Polycomb Repressive Complex 2 (PRC2) is a histone methyltransferase complex composed of core subunits Ezh2 (or Ezh1), Eed, Suz12 and Rbbp4. PRC2 trimethylates histone H3K27 (H3K27me3) to mark developmentally repressed chromatin. Ezh2 contains a split catalytic region composed of the SET domain and the SET Activation Loop (SAL) but is inactive without minimally associating with Eed and the VEFS domain of Suz12 [Suz12(VEFS)]4–8. Pyridone inhibitors bind to Ezh2 in an extended pocket that overlaps with the SAM binding site.

To obtain a more holistic understanding of PRC2 inhibition by pyridone inhibitors, we attempted to solve crystal structures of human PRC2 in complex with inhibitors that had not been previously characterized. We established a system to co-express a fusion of full length Ezh2 and [Suz12(VEFS)] with full length Eed in S. cerevisiae, and further engineered Ezh2 by deleting amino acids 183–195 and 341–427 to produce diffracting crystals (protein purity in Fig. S2A). Although the resolution of the crystal structure is limited to 3.9 Å, Fo − Fc difference electron density for GSK126 was clear enough to build the drug into the structure. Continuous electron density is observed for the body of the drug, while the tail, arm, and head regions are partially resolved to varying degrees. The top, right-hand side of the drug-binding pocket (relative to the pyridone moiety at top) is formed by residues W624, R685, and F686. In a manner similar to other pyridone inhibitors, the amide nitrogen and carbonyl oxygen of the pyridone head of GSK126 mediate distorted hydrogen bonds with the main chain carbonyl oxygen and amide nitrogen, respectively, of residue W624 of Ezh2 to compete with SAM binding to the same residue. Residues I109, M110 and Y111 of the SAL of Ezh2 form the bottom of the binding pocket. The backbone carbonyl oxygen on the neck region between the pyridone and the indole moieties of the drug binds to the backbone amide nitrogen of residue Y111, and the side chain of Y111 interacts with the indole body moiety. The left-hand side of the pocket is formed by residues 661–665 of the SET domain, and this region constricts access to the pocket. Residues Y661 and Y111 form a gating region in a manner similar to other PRC2 structures.

>SNAHHHHHHGQTGKKSEKGPVCWRKRVKSEYMRLRQLKRFRRADEVKSMFSSNRQKILERTEILNQEWKQRRIQPVHILTSVSSLRGTRECSVTSDLDFPTQVIPLKTLNAVASVPIMYSWSPLQQNFMVEDETVLHNIPYMGDEVLDQDGTFIEELIKNYDGKVHGDRECGFINDEIFVELVNALGQYNREEKQKDLEDHRDDKESRPPRKFPSDKIFEAISSMFPDKGTAEELKEKYKELTEQQLPGALPPECTPNIDGPNAKSVQREQSLHSFHTLFCRRCFKYDCFLHPFHATPNTYKRKNTETALDNKPCGPQCYQHLEGAKEFAAALTAERIKTPPKRPGGRRRGRLPNNSSRPSTPTINVLESKDTDSDREAGKPNIEPPENVEWSGAEASMFRVLIGTYYDNFCAIARLIGTKTCRQVYEFRVKESSIIAPAPAEDVDTPPRKKKRKHRLWAAHCRKIQLKKDGSSNHVYNYQPCDHPRQPCDSSCPCVIAQNFCEKFCQCSSECQNRFPGCRCKAQCNTKQCPCYLAVRECDPDLCLTCGAADHRDSKNVSCKNCSIQRGSKKHLLLAPSDVAGWGIFIKDPVQKNEFISEYCGEIISQDEADRRGKVYDKYMCSFLFNLNNDFVVDATRKGNKIRFANHSVNPNCYAKVMMVNGDHRIGIFAKRAIQTGEELFFDYRYSQADALKYVGIEREMEIPFLESEDGEVEQQRTYSSGHNRLYFHSDTCLPLRPQEMEVDSEDEKDPEWLREKTITQIEEFSDVNEGEKEVMKLWNLHVMKHGFIADNQMNHACMLFVENYGQKIIKKNLCRNFMLHLVSMHDFNLISIMSIDKAVTKLREMQQKLEKGESAS[2x];>[2x]MSSEREVSTAPAGTDMPAAKKQKLSSDENSNPDLSGDENDDAVSIESGTNTERPDTPTNTPNAPGRKSWGKGKWKSKKCKYSFKCVNSLKEDHNQPLFGVQFNWHSKEGDPLVFATVGSNRVTLYECHSQGEIRLLQSYVDADADENFYTCAWTYDSNTSHPLLAVAGSRGIIRIINPITMQCIKHYVGHGNAINELKFHPRDPNLLLSVSKDHALRLWNIQTDTLVAIFGGVEGHRDEVLSADYDLLGEKIMSCGMDHSLKLWRINSKRMMNAIKESYDYNPNKTNRPFISQKIHFPDFSTRDIHRNYVDCVRWLGDLILSKSCENAIVCWKPGKMEDDIDKIKPSESNVTILGRFDYSQCDIWYMRFSMDFWQKMLALGNQVGKLYVWDLEVEDPHKAKCTTLTHHKCGAAIRQTSFSRDSSILIAVCDDASIWRWDRLR> GHMSRHDVTNATLETTGKELTETYMEMLNGDVVEVSIANEERIVSLLSSLASANVTLKQLIGTKIGVAVGQFLSDGFPPHIVRFSKGILD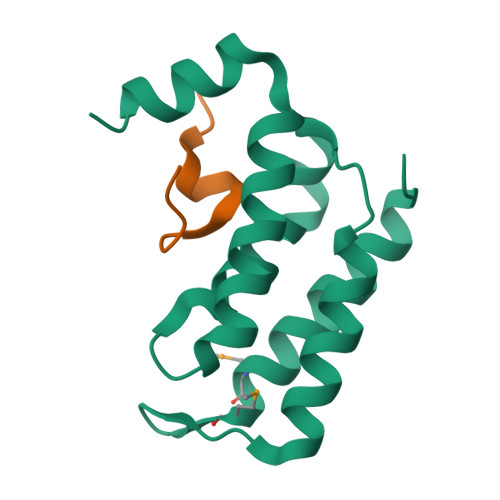YWFRQLPEEVQKQLLAKRALG;> GSTLEDLFGPLFYVDKSL>[5x]GQDMVSPPPPIADEPLTVNTGIYLIECYSLDDKAETFKVNAFLSLSWKDRRLAFDPVRSGVRVKTYEPEAIWIPEIRFVNVANARDADVVDISVSPDGTVQYLERFSARVLSPLDFRRYPFDSQTLHIYLIVRSVDTRNIVLAVDLEKVGKNDDVFLTGWDIESFTAVVKPANFALEDRLESKLDYQLRISRQYFSYIPNIILPMLFILFISWTAFWSTS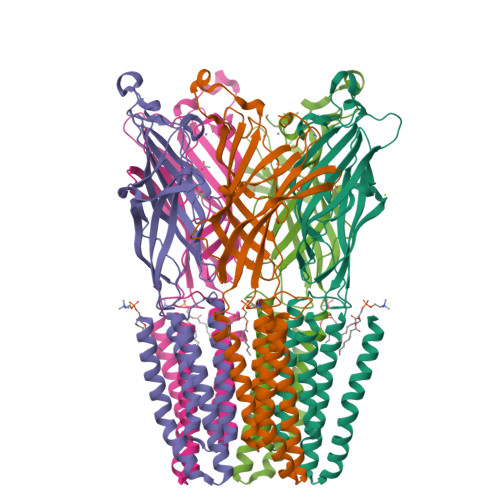YEANVTLVVSTLIAHIAFNILVETNLPKTPYMTYTGAIIFMIYLFYFVAVIEVTVQHYLKVESQPARAASITRASRIAFPVVFLLANIILAFLFFGF> GLQGHIIENPQ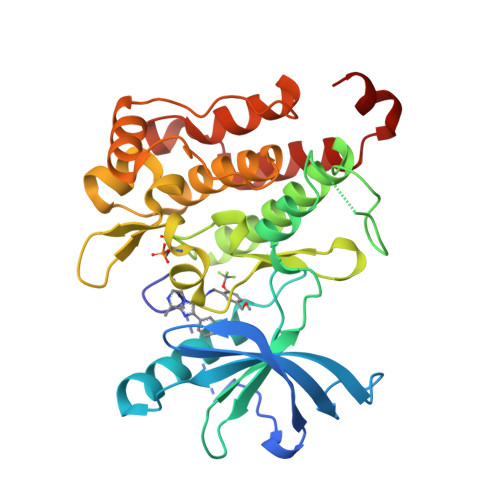YFSDACVHHIKRRDIVLKWELGEGAFGKVFLAECHNLLPEQDKMLVAVKALKEASESARQDFQREAELLTMLQHQHIVRFFGVCTEGRPLLMVFEYMRHGDLNRFLRSHGPDAKLLAGGEDVAPGPLGLGQLLAVASQVAAGMVYLAGLHFVHRDLATRNCLVGQGLVVKIGDFGMSRDIYSTDYYRVGGRTMLPIRWMPPESILYRKFTTESDVWSFGVVLWEIFTYGKQPWYQLSNTEAIDCITQGRELERPRACPPEVYAIMRGCWQREPQQRHSIKDVHARLQALAQAPPVYLDVL> MAFARGGLAQTASQTTSSPVRVGLSVDAS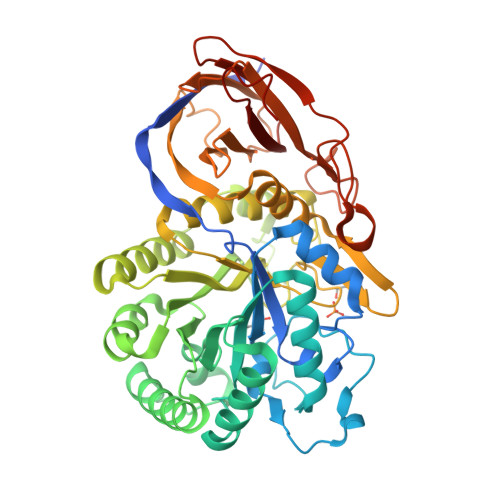ALGHTIPPDYTGLSYEQAQMANPNYFSGANTQLAGFLRTLGRQGVLRIGGNTSEYTFWNRHAKPTAADEHLAAGPDKGHHAAAREVITPEAVNNLSEFLDKTGWKLIYGLNLGKGTPENAADEAAYVMETIGADRLLAFQLGNEPDLFYRNGIRPASYDFAAYAGDWQRFFTAIRKRVPNAPFAGPDTAYNTKWLVPFADKFKHDVKFISSHYYAEGPPTDPSMTIERLMKPNPRLLGETAGLKQVEADTGLPFRLTETNSCYQGGKQGVSDTFAAALWAGDLMYQQAAAGSTGINFHGGGYGWYTPVAGTPEDGFIARPEYYGMLLFAQAGAGQLLGAKLTDNSAAPLLTAYALRGTDGRTRIALFNKNLDADVEVAISGVASPSGTVLRLEAPRADDTTDVTFGGAPVGASGSWSPLVQEYVPGHSGQFVLHMRKASGALLEFAKLAAALQHHHHHH>MEQPGLCGLSNLGN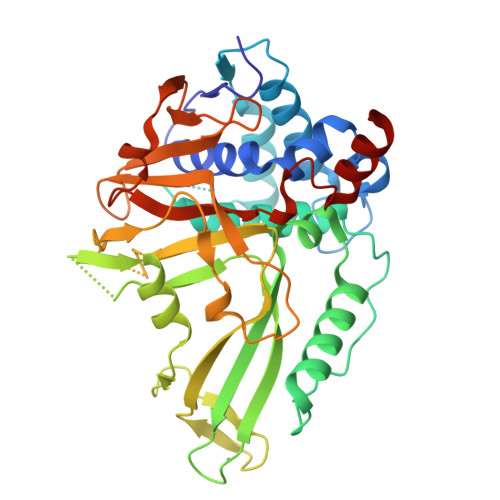TCFMNSAIQCLSNTPPLTEYFLNDKYQEELNFDNPLGMRGEIAKSYAELIKQMWSGKFSYVTPRAFKTQVGRFAPQFSGYQQQDCQELLAFLLDGLHEDLNRIRKKPYIQLKDADGRPDKVVAEEAWENHLKRNDSIIVDIFHGLFKSTLVCPECAKISVTFDPFCYLTLPLASTSKVKLKDCIELFTTKEKLGAEDPWYCPNCKEHQQATKKLDLWSLPPVLVVHLKRFSYSRYMRDKLDTLVDFPINDLDMSEFLINPNAGPCRYNLIAVSNHYGGMGGGHYTAFAKNKDDGKWYYFDDSSVSTASEDQIVSKAAYVLFYQRQDTFSGTGFFPLDRETLEHHHHHH[2x]>[2x]MSKVPVVGIVAALLPEMG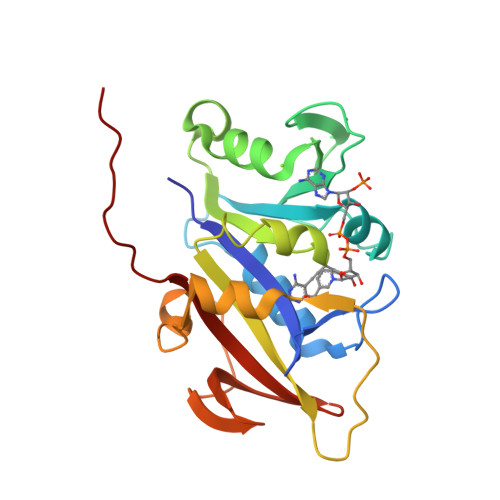IGFQGNLPWRLAKEMKYFREVTTLTNDNSKQNVVIMGRKTWESIPQKFRPLPKRINVVVSRSFDGELRKVEDGIYHSNSLRNCLTALQSSLANENKIERIYIIGGGEIYRQSMDLADHWLITKIMPLPETTIPQMDTFLQKQELEQRFYDNSDKLVDFLPSSIQLEGRLTSQEWNGELVKGLPVQEKGYQFYFTLYTKKLEHHHHHHHH>MGSSHHHHHHHHSSGLVPRGSHMFYPDPFDVIIIGGGHAGTEAAMAAARMGQQTLLLTHNIDTLGQMSCNPAIGGIGKGHLVKEVDALGGLMAKAIDQAGIQFRILNASKGPAVRATRAQADRVLYRQAVRTALENQPNLMIFQQAVEDLIVENDRVVGAVTQMGLKFRAKAVVLTVGTFLDGKIHIGLDNYSGGRAGDPPSIPLSRRLRELPLRVGRLKTGTPPRI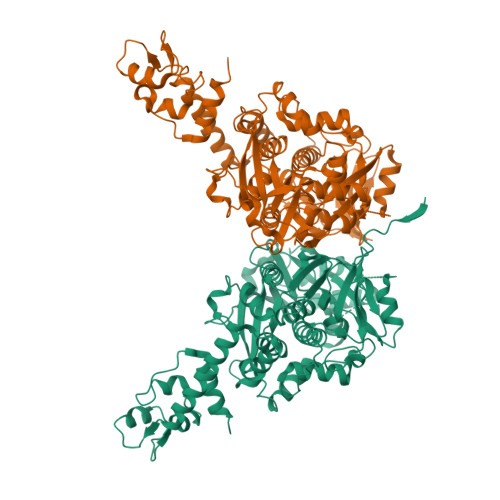DARTIDFSVLAQQHGDNPMPVFSFMGNASQHPQQVPCYITHTNEKTHDVIRSNLDRSPMYAGVIEGVGPRYCPSIEDKVMRFADRNQHQIFLEPEGLTSNEIYPNGISTSLPFDVQMQIVRSMQGMENAKIVRPGYAIEYDFFDPRDLKPTLESKFIQGLFFAGQINGTTGYEEAAAQGLLAGLNAARLSADKEGWAPARSQAYLGVLVDDLCTLGTKEPYRMFTSRAEYRLMLREDNADLRLTEIGRELGLVDDERWARFNEKLENIERERQRLKSTWVTPSAEAAAEVNAHLTAPLSREASGEDLLRRPEMTYEKLTTLTPFAPALTDEQAAEQVEIQVKYEGYIARQQDEIEKQLRNENTLLPATLDYRQVSGLSNEVIAKLNDHKPASIGQASRISGVTPAAISILLVWLKKQGMLRRSA[4x]>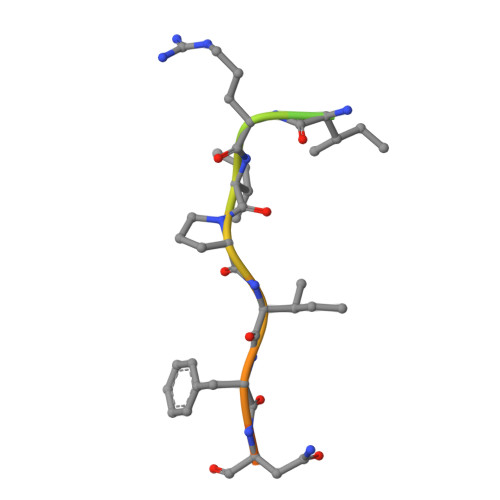 ADISVLPEIRIPIFNSLKMQ> MSSMILTQFRPFIESISGITDQSNDVFEDAAKAFSMFTRSDVYKALDEIPFSDDAMLPIPPTIYTKPSHDSYYYIDALNRVRRKTYQGPDDVYVPNCSIVELLEPHETLTSYGRLSEAIENRAKDGDSQARIATTYGRIAESQARQIKAPLEKFVLALLVSEAGGSLYDPVLQKYDEIPDLSHNCPLWCFREICRHISGPLPDRAPYLYLSAGVFWLMSPRMTSAIPPLLSDLVNLAILQQTAGLDPSLVKLGVQICLHAAASSSYAWFILKTKSIFPQNTLHSMYESLEGGYCPNLEWLEPRSDYKFMYMGVMPLSTKYARSAPSNDKKARELGEKYGLSSVVSELRKRTKTYVKHDFASVRYIRDAMACTSGIFLVRTPTETVLQEYTQSPEIKVPIPQKDWTGPVGEIRILKDTTSSIARYLYRTWYLAAARMAAQPRTWDPLFQAIMRSQYVTARGGSGAALRESLYAINVSLPDFKGLPVKAATKIFQAAQLANLPFSHTSVAILADTSMGLRNQVQRRPRSIMPLNVPQQQVSAPHTLTADYINYHMNLSTTSGSAVIEKVIPLGVYASSPPNQSINIDISACDASITWDFFLSVIMAAIHEGVASGSIGKPFMGVPASIVNDESVVGVRAARPISGMQNMIQHLSKLYKRGFSYRVNDSFSPGNDFTHMTTTFPSGSTATSTEHTANNSTMMETFLTVWGPEHTDDPDVLRLMKSLTIQRNYVCQGDDGLMIIDGNTAGKVNSETIQKMLELISKYGEEFGWKYDIAYDGTAEYLKLYFIFGCRIPNLSRHPIVGKERANSSAEEPWPAILDQIMGIFFNGVHDGLQWQRWIRYSWALCCAFSRQRTMIGESVGYLQYPMWSFVYWGLPLVKVFGSDPWIFSWYMPTGDLGMYSWISLIRPLMTRWMVANGYATDRCSPVFGNADYRRCFNEIKLYQGYYMAQLPRNPTKSGRAAPREVREQFTQALSDYLMQNPELKSRVLRGRSEWEKYGAGIIHNPPSLFDVPHKWYLGAQEAATATREELAEMDETLMRARRHSYSSFSKLLEAYLLVKWRMCEAREPSVDLRLPLCAGIDPLNSDPFLKMVSVGPMLQSTRKYFAQTLFMAKTVSGLDVNAIDSALLRLRTLGADKKALTAQLLMVGLQESEADALAGKIMLQDVSTVQLARVVNLAVPDTWMSLDFDSMFKHHVKLLPKDGRHLNTDIPPRMGWLRAILRFLGAGMVMTATGVAVDIYLEDIHGGGRALGQRFMTWMRQEGRSA;>MGNASSIVQTINVTGDGNVFKPSAETSSTAVPSLSLSPGMLNPGGVPWIAIGDETSVTSPGALRRMTSKDIPETAIINTDNSSGAVPSESALVPYNDEPLVVVTEHAIANFTKAEMALEFNREFLDKLRVLSVSPKYSDLLTYVDCYVGVSARQALNNFQKQVPVITPTRQTMYVDSIQAALKALEKWEIDLRVAQTLLPTNVPIGEVSCPMQSVVKLLDDQLPDDSLIRRYPKEAAVALAKRNGGIQWMDVSEGTVMNEAVNAVAASALAPSASAPPLEEKSKLTEQAMDLVTAAEPEIIASLVPVPAPVFAIPPKPADYNVRTLKIDEATWLRMIPKTMGTLFQIQVTDNTGTNWHFNLRGGTRVVNLDQIAPMRFVLDLGGKSYKETSWDPNGKKVGFIVFQSKIPFELWTAASQIGQATVVNYVQLYAEDSSFTAQSIIATTSLAYNYEPEQLNKTDPEMNYYLLATFIDSAAITPTNMTQPDVWDALLTMSPLSAGEVTVKGAVVSEVVPAELIGSYTPESLNASLPNDAARCMIDRASKIAEAIKIDDDAGPDEYSPNSVPIQGQLAISQLETGYGVRIFNPKGILSKIASRAMQAFIGDPSTIITQAAPVLSDKNNWIALAQGVKTSLRTKSLSAGVKTAVSKLSSSESIQNWTQGFLDKVSTHFPAPKPDCPTNGDGSEPSARRVKRDSYAGVVKRGYTR[10x];>MEVCLPNGHQIVDLINNAFEGRVSIYSAQEGWDKTISAQPDMMVCGGAVVCMHCLGVVGSLQRKLKHLPHHRCNQQIRHQDYVDVQFADRVTAHWKRGMLSFVCQMHAMMNDVSPEDLDRVRTEGGSLVELNWLQVDPNSMFRSIHSSWTDPLQVVDDLDTKLDQYWTALNLMIDSSDLVPNFMMRDPSHAFNGVRLEGDARQTQFSRTFDSRSSLEWGVMVYDYSELEHDPSKGRAYRKELVTPARDFGHFGLSHYSRATTPILGKMPAVFSGMLTGNCKMYPFIKGTAKLKTVRKLVDSVNHAWGVEKIRYALGPGGMTGWYNRTMQQAPIVLTPAALTMFSDTTKFGDLDYPVMIGDPMILG[10x];> MANVWGVRLADSLSSPTIETRTRQYTLHDLCSDLDANPGREPWKPLRNQRTNNIVAVQLFRPLQGLVLDTQLYGFPGAFDDWERFMREKLRVLKYEVLRIYPISNYSNEHVNVFVANALVGAFLSNQAFYDLLPLLIINDTMIGDLLGTGASLSQFFQSHGDVLEVAAGRKYLQMENYSNDDDDPPLFAKDLSDYAKAFYSDTYEVLDRFFWTHDSSAGVLVHYDKPTNGHHYLLGTLTQMVSAPPYIINATDAMLLESCLEQFSANVRARPAQPVTRLDQCYHLRWGAQYVGEDSLTYRLGVLSLLATNGYQLARPIPRQLTNRWLSSFVSQIMSDGVNETPLWPQERYVQIAYDSPSVVDGATQYGYVRKNQLRLGMRISALQSLSDTPSPVQWLPQYTIDQAAMDEGDLMVSRLTQLPLRPDYGNIWVGDALSYYVDYNRSHRVVLSSELPQLPDTYFDGDEQYGRSLFSLARKIGDRSLVKDTAVLKHAYQAIDPNTGKEYLRSRQSVAYFGASAGHSGADQPLVIEPWIQGKISGVPPPSSVRQFGYDVARGAIVDLARPFPSGDYQFVYSDVDQVVDGHDDLSISSGLVESLLSSCMHATAPGG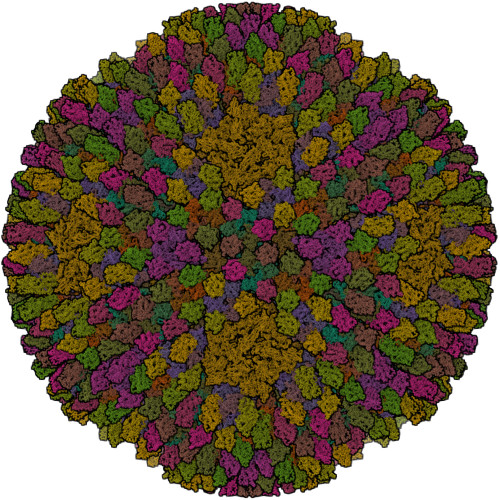SFVVKINFPTRPVWHYIEQKILPNITSYMLIKPFVTNNVELFFVAFGVHQHSSLTWTSGVYFFLVDHFYRYETLSTISRQLPSFGYVDDGSSVTGIETISIENPGFSNMTQAARIGISGLCANVGNARKSIAIYESHGARVLTITSRRSPASARRKSRLRYLPLIDPRSLEVQARTILPADPVLFENVSGASPHVCLTMMYNFEVSSAVYDGDVVLDLGTGPEAKILELIPATSPVTCVDIRPTAQPSGCWNVRTTFLELDYLSDGWITGVRGDIVTCMLSLGAAAAGKSMTFDAAFQQLIKVLSKSTANVVLVQVNCPTDVVRSIKGYLEIDSTNKRYRFPKFGRDEPYSDMDALEKICRTAWPNCSITWVPLSYDLRWTRLALLESTTLSSASIRIAELMYKYMPIMRIDIHGLPMEKRGNFIVGQNCSLVIPGFNAQDVFNCYFNSALAFSTEDVNAAMIPQVSAQFDATKGEWTLDMVFSDAGIYTMQALVGSNANPVSLGSFVVDSPDVDITDAWPAQLDFTIAGTDVDITVNPYYRLMTFVRIDGQWQIANPDKFQFFSSASGTLVMNVKLDIADKYLLYYIRDVQSRDVGFYIQHPLQLLNTITLPTNEDLFLSAPDMREWAVKESGNTICILNSQGFVLPQDWDVLTDTISWSPSIPTYIVPPGDYTLTPL;>MKRIPRKTKGKSSGKGNDSTERSDDGSSQLRDKQNNKAGPATTEPGTSNREQYRARPGIASVQRATESAELPMKNNDEGTPDKKGNTRGDLVNEHSEAKDEADEATQKQAKDTDKSKAQVTYSDTGINNANELSRSGNVDNEGGSNQKPMSTRIAEATSAIVSKHPARVGLPPTASSGHGYQCHVCSAVLFSPLDLDAHVASHGLHGNMTLTSSEIQRHITEFISSWQNHPIVQVSADVENKKTAQLLHADTPRLVTWDAGLCTSFKIVPIVPAQVPQDVLAYTFFTSSYAIQSPFPEAAVSRIVVHTRWASNVDFDRDSSVIMAPPTENNIHLFKQLLNTETLSVRGANPLMFRANVLHMLLEFVLDNLYLNRHTGFSQDHTPFTEGANLRSLPGPDAEKWYSIMYPTRMGTPNVSKICNFVASCVRNRVGRFDRAQMMNGAMSEWVDVFETSDALTVSIRGRWMARLARMNINPTEIEWALTECAQGYVTVTSPYAPSVNRLMPYRISNAERQISQIIRIMNIGNNATVIQPVLQDISVLLQRISPLQIDPTIISNTMSTVSESTTQTLSPASSILGKLRPSNSDFSSFRVALAGWLYNGVVTTVIDDSSYPKDGGSVTSLENLWDFFILALALPLTTDPCAPVKAFMTLANMMVGFETIPMDNQIYTQSRRASAFSTPHTWPRCFMNIQLISPIDAPILRQWAEIIHRYWPNPSQIRYGAPNVFGSANLFTPPEVLLLPIDHQPANVTTPTLDFTNELTNWRARVCELMKNLVDNQRYQPGWTQSLVSSMRGTLDKLKLIKSMTPMYLQQLAPVELAVIAPMLPFPPFQVPYVRLDRDRVPTMVGVTRQSRDTITQPALSLSTTNTTVGVPLALDARAITVALLSGKYPPDLVTNVWYADAIYPMYADTEVFSNLQRDMITCEAVQTLVTLVAQISETQYPVDRYLDWIPSLRASAATAATFAEWVNTSMKTAFDLSDMLLEPLLSGDPRMTQLAIQYQQYNGRTFNVIPEMPGSVIADCVQLTAEVFNHEYNLFGIARGDIIIGRVQSTHLWSPLAPPPDLVFDRDTPGVHIFGRDCRISFGMNGAAPMIRDETGMMVPFEGNWIFPLALWQMNTRYFNQQFDAWIKTGELRIRIEMGAYPYMLHYYDPRQYANAWNLTSAWLEEITPTSIPSVPFMVPISSDHDISSAPAVQYIISTEYNDRSLFCTNSSSPQTIAGPDKHIPVERYNILTNPDAPPTQIQLPEVVDLYNVVTRYAYETPPITAVVMGVP[2x];>MARAAFLFKTVGFGGLQNVPINDELSSHLLRAGNSPWQLTQFLDWISLGRGLATSALVPTAGSRYYQMSCLLSGTLQIPFRPNHRWGDIRFLRLVWSAPTLDGLVVAPPQVLAQPALQAQADRVYDCDDYPFLARDPRFKHRVYQQLSAVTLLNLTGFGPISYVRVDEDMWSGDVNQLLMNYFGHTFAEIAYTLCQASANRPWEHDGTYARMTQIILSLFWLSYVGVIHQQNTYRTFYFQCNRRGDAAEVWILSCSLNHSAQIRPGNRSLFVMPTSPDWNMDVNLILSSTLTGCLCSGSQLPLIDNNSVPAVSRNIHGWTGRAGNQLHGFQVRRMVTEFCDRLRRDGVMTQAQQNQIEALADQTQQFKRDKLEAWAREDDQYNQANPNSTMFRTKPFTNAQWGRGNTGATSAAIAALI[3x]>[2x]MHHHHHHGSENLYFQGSKFSAKRLPSTRLGTFLENRVNDFLRRQNHPESGEVTVRVVHASDKTVEVKPGMKARFVDSGEMAESFPYRTKALFAFEEIDGVDLCFFGMHVQEYGSDCPPPNQRRVYISYLDSVHFFRPKCLRTAVYHEILIGYLEYVKKLGYTTGHIWACPPSEGDDYIFHCHPPDQKIPKPKRLQEWFKKMLDKAVSERIVHDYKDIFKQATEDRLTSAKELPYFEGDFWPNVLEESIKESGGSGSQKLYATMEKHKEVFFVIRLIAGPAANSLPPIVDPDPLIPCDLMDGRDAFLTLARDKHLEFSSLRRAQWSTMCMLVELHTQSQ

P300 is an ∼2400AA multidomain protein whose catalytic core consists of bromo-, RING, PHD, and histone acetyltransferase (HAT) domains. By acetylating histones, p300 promotes gene expression. It can also acetylate itself, as well as other proteins, and recruit a larger complex of proteins including transcription factors. The overall structure is as expected from previous p300-HAT structures: a central β-sheet is composed of seven β-strands and surrounded by nine α-helices.

To improve homogeneity, a construct omitting the autoacetylation-prone autoinhibitory loop was inactivated through mutation of residue Y1467 to F: p300‐HAT‐YF‐Δloop [K1287‐Q1663/Y1467F/Δ(L1520‐L1580)] and overexpressed in E. coli. Ternary crystals of p300‐HAT‐YF‐Δloop with CoA and CPI-090 were obtained at 4° C from 200 + 150 nl sitting drops with a 60 μL reservoir consisting of 0.1 M CHES pH 9.5 and 30% w/v PEG 3000 [MCSG1 (MCSG) (purchased from Anatrace), condition A2]. Followup with dynamic scanning fluorimetry (DSF) of the P300-HAT domain indicated strong stabilization, especially for CPI-090. Despite their chemical differences, these new allosteric compounds bind in the same location, ∼8 Å distant from the active site, between the α5 and α6 helices. There are few structural differences between these ternary compound/CoA/HAT structures and CoA/HAT binary structures. Essentially, the allosteric compounds displace water molecules. However, derivatization failed to improve the compound activity from this starting point (data not shown). The indole compound CPI-090, a stronger HAT inhibitor at 0.31 μM, offered vectors for optimization from the 4, 5, and 6 positions of its pyridine ring [Fig. 6(b)]. Derivatization yielded actionable SAR and improvement in the biochemical activity (data not shown), and so this series was selected for cell-based assays. CPI-090 does not inhibit the FL enzyme in our experiments.> MKQIKAHLTRYLEEILKLSSQEYLTEFVQLGIEELAWGERKIPEKLKGAIIDTY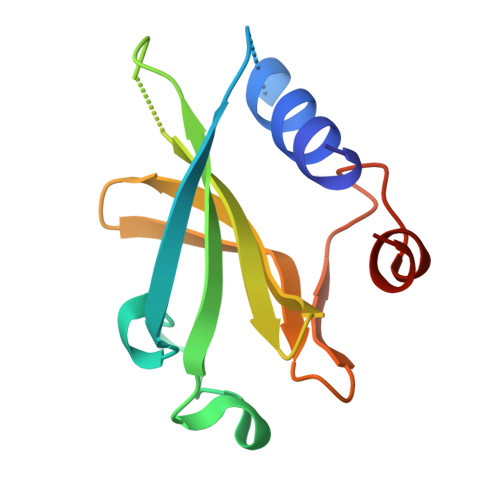TFYDHSLIKDYIYSFIGTYQGKIILVGYTNGEYEHFFYINDTVKTLHSELHLLNLTEEDLEFVNVG>[2x]EENFSRSYPCDEKKQNDSVIAECSNRRLQEVPQTVGKYVTELDLSDNFITHITNESFQGLQNLTKINLNHNPNVQHQNGNPGIQSNGLNITDGAFLNLKNLRELLLEDNQLPQIPSGLPESLTELSLIQNNIYNITKEGISRLINLKNLYLAWNCYFNKVCEKTNIEDGVFETLTNLELLSLSFNSLSHVPPKLPSSLRKLFLSNTQIKYISEEDFKGLINLTLLDLSGNC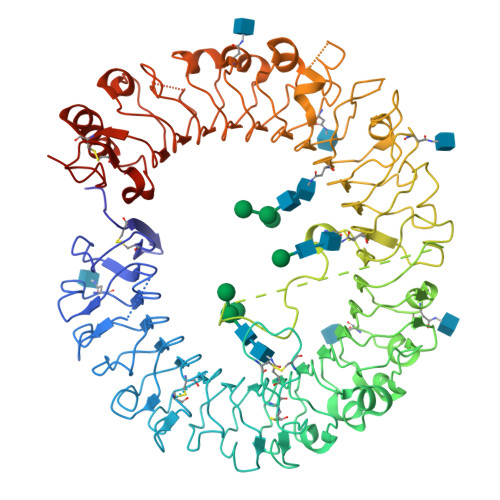PRCFNAPFPCVPCDGGASINIDRFAFQNLTQLRYLNLSSTSLRKINAAWFKNMPHLKVLDLEFNYLVGEIASGAFLTMLPRLEILDLSFNYIKGSYPQHINISRNFSKLLSLRALHLRGYVFQELREDDFQPLMQLPNLSTINLGINFIKQIDFKLFQNFSNLEIIYLSENRISPLVKDTRQSYANSSSFQRHIRKRRSTDFEFDPHSNFYHFTRPLIKPQCAAYGKALDLSLNSIFFIGPNQFENLPDIACLNLSANSNAQVLSGTEFSAIPHVKYLDLTNNRLDFDNASALTELSDLEVLDLSYNSHYFRIAGVTHHLEFIQNFTNLKVLNLSHNNIYTLTDKYNLESKSLVELVFSGNRLDILWNDDDNRYISIFKGLKNLTRLDLSLNRLKHIPNEAFLNLPASLTELHINDNMLKFFNWTLLQQFPRLELLDLRGNKLLFLTDSLSDFTSSLRTLLLSHNRISHLPSGFLSEVSSLKHLDLSSNLLKTINKSALETKTTTKLSMLELHGNPFECTCDIGDFRRWMDEHLNVKIPRLVDVICASPGDQRGKSIVSLELTTCVSDVTEFLVPR> MSPFPLTSMDKAFITVLEMTPVLGTEIINYRDGMGRVLAQDVYAKDNLPPFPASVKDGYAVRAADGPGDRFIIGESQAGEQPTQTVMPGQVMRVTTGAPIPCGADAVVQVEDTELIRESDDGTEELEVRILVQARPGQDIRPIGHDIKRGECVLAKGTHMGPSEIGLLATVGVTEVEVNKFPVVAVMSTGNELLNPEDDLLPGKIRDSNRSTLLATIQEHGYPTINLGIVGDNPDDLLNALNEGISRADVIITSGGVSMGEKDYLKQV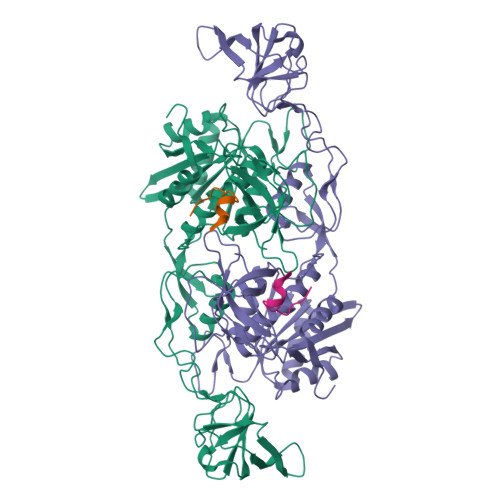LDIDLHAQIHFGRVFMKPGLPTTFATLDIDGVRKIIFALPGNPVSAVVTCNLFVVPALRKMQGILDPRPTIIKARLSCDVKLDPRPEYHRCILTWHHQEPLPWAQSTGNQMSSRLMSMRSANGLLMLPPKTEQYVELHKGEVVDVMVIGRL;> FSIVGSLPRDFEL> GSIHVISRDQSTPIIEVEGPLLSDTHVTFKLTMPSPMPEYLNVHYICESASRLLFLSMHWARSIPAFQALGQDCNTSLVRACWNELFTLG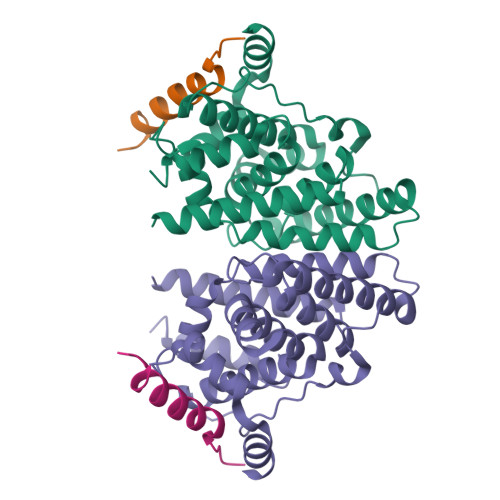LAQCAQVMSLSTILAAIVNHLQNSIQEDKLSGDRIKQVMEHIWKLQEFCNSMAKLDIDGYEYAYLKAIVLFSPDHPGLTSTSQIEKFQEKAQMELQDYVQKTYSEDTYRLARILVRLPALRLMSSNITEELFFTGLIGNVSIDSIIPYILKMETAEYNGQITGASL;> QQPTYVALSYINRFMTDAARREQES>[2x]MA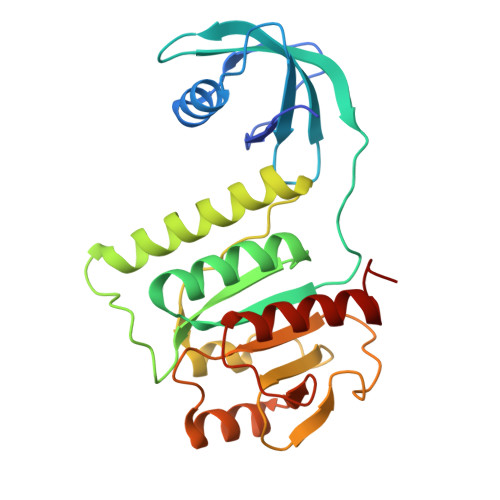HHHHHHMPRFYLPENLSVGQTVDLPDNIVRHLNVLRVRPNENITLFDGKGKAHTARLTVLEKHRAEAEILHEDTTDNESPLNITLIQSISSGDRMDFTLQKSVELGVTAIQPVISERCIVRLDGERAAKRLARWQEIVISACEQSGRNTVPPVLPIIGYREALDKMPSENTKLIMSINRACKLGDIRHPSGAIVFMVGPEGGWTEQEEQQAFEAGFQAVTLGKRILRTETAPLAAIAAMQTLWGDFT2-(2-PHENYL-3-PYRIDIN-2-YL-4,5,6,7-TETRAHYDRO-2H-ISOPHOSPHINDOL-1-YL)PYRIDINE | C24 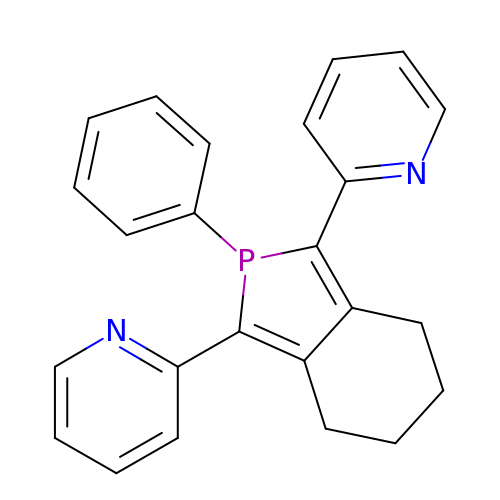H21 N2 P | GSKNNHAAFLPYHG-UHFFFAOYSA-N> MSADAQSFLNRVCGVSAARLTPCGTGTSTDVVYRAFDIYNDKVAGFAKFLKTNCCRFQEKDEDDNLIDSYFVVKRHTFSNYQHEETIYNLLKDCPAVAKHDFFKFRIDGDMVPHISRQRLTKYTMADLVYALRHFDEGNCDTLKEILVTYNCCDDDYFNKKDWYDFVENPDILRVYANLGERVRQALLKTVQFCDAMRNAGIVGVLTLDNQDLNGNWYDFGDFIQTTPGSGVPVVDSYYSLLMPILTLTRALTAESHVDTDLTKPYIKWDLLKYDFTEERLKLFDRYFKYWDQTYHPNCVNCLDDRCILHCANFNVLFSTVFPPTSFGPLVRKIFVDGVPFVVSTGYHFRELGVVHNQDVNLHSSRLSFKELLVYAADPAMHAASGNLLLDKRTTCFSVAALTNNVAFQTVKPGNFNKDFYDFAVSKGFFKEGSSVELKHFFFAQDGNAAISDYDYYRYNLPTMCDIRQLLFVVEVVDKYFDCYDGGCINANQVIVNNLDKSAGFPFNKWGKARLYYDSMSYEDQDALFAYTKRNVIPTITQMNLKYAISAKNRARTVAGVSICSTMTNRQFHQKLLKSIAATRGATVVIGTSKFYGGWHNMLKTVYSDVENPHLMGWDYPKCDRAMPNMLRIMASLVLARKHTTCCSLSHRFYRLANECAQVLSEMVMCGGSLYVKPGGTSSGDATTAYANSVFNICQAVTANVNALLSTDGNKIADKYVRNLQHRLYECLYRNRDVDTDFVNEFYAYLRKHFSMMILSDDAVVCFNSTYASQGLVASIKNFKSVLYYQNNVFMSEAKCWTETDLTKGPHEFCSQHTMLVKQGDDYVYLPYPDPSRILGAGCFVDDIVKTDGTLMIERFVSLAIDAYPLTKHPNQEYADVFHLYLQYIRKLHDELTGHMLDMYSVMLTNDNTSRYWEPEFYEAMYTPHTVLQGGSENLYFQGHHHHHHHH;>MAIASEFSSLPSYAAFATAQEAYEQAVANGDSEVVLKKLKKSLNVAKSEFDRDAAMQRKLEKMADQAMTQMYKQARSEDKRAKVTSAM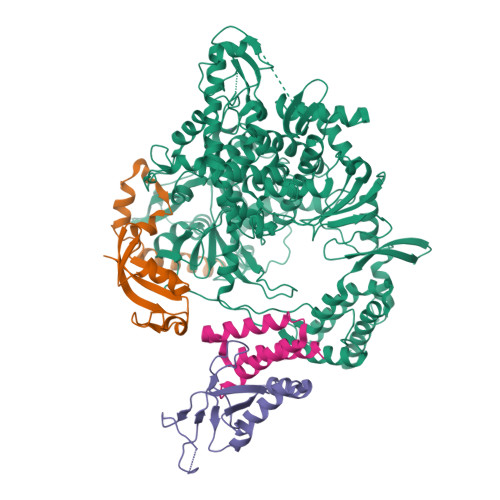QTMLFTMLRKLDNDALNNIINNARDGCVPLNIIPLTTAAKLMVVIPDYNTYKNTCDGTTFTYASALWEIQQVVDADSKIVQLSEISMDNSPNLAWPLIVTALRANSAVKLQHHHHHHHH[2x];> MSKMSDVKCTSVVLLSVLQQLRVESSSKLWAQCVQLHNDILLAKDTTEAFEKMVSLLSVLLSMQGAVDINKLCEEMLDNRATLQHHHHHHHH> IHRDLKPS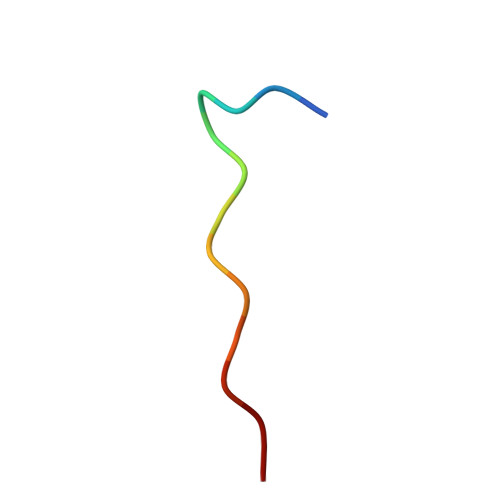NLLIN> MNLLVTSSLGVLLHLVVLCQADDHSELLVNTKSGKVMGTRVPVLSSHISAFLGIPFAEPPVGNMRFRRPEPKKPWSGVWNASTYPNNCQQYVDEQFPGFSGSEMWNPNREMSEDCLYLNIWVPSPRPKSTTVMVWIYGGGFYSGSSTLDVYNGKYLAYTEEVVLVSLSYRVGAFGFLALHGSQEAPGNVGLLDQRMALQWVHDNIQFFGGDPKTVTIFGESAGGASVGMHILSPGSRDLFRRAILQSGSPNCPWASVSVAEGRRRAVELGRNLNCNLNSDEELIHCLREKKPQELIDVEWNVLPFDSIFRFSFVPVIDGEFFPTSLESMLNSGNFKKTQILLGVNKDEGSFFLLYGAPGFSKDSESKISREDFMSGVKLSVPHANDLGL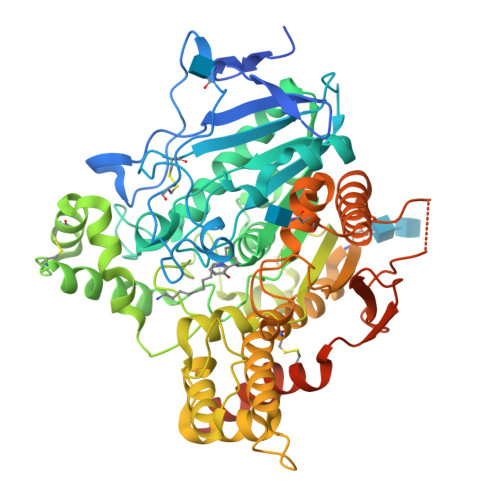DAVTLQYTDWMDDNNGIKNRDGLDDIVGDHNVICPLMHFVNKYTKFGNGTYLYFFNHRASNLVWPEWMGVIHGYEIEFVFGLPLVKELNYTAEEEALSRRIMHYWATFAKTGNPNEPHSQESKWPLFTTKEQKFIDLNTEPMKVHQRLRVQMCVFWNQFLPKLLNATACDGELSSSGTSSSKGIIFYVLFSILYLIF> GSHMSDNPKVLVADDDKKIAQFIKTKFEENGIDTTVAFDGKEALFLINTNNYDVIVIDWMMPYLDGISLLKILRKQNINTPVIILSALDSTENKIEGLKSGSDDYLTKPFSID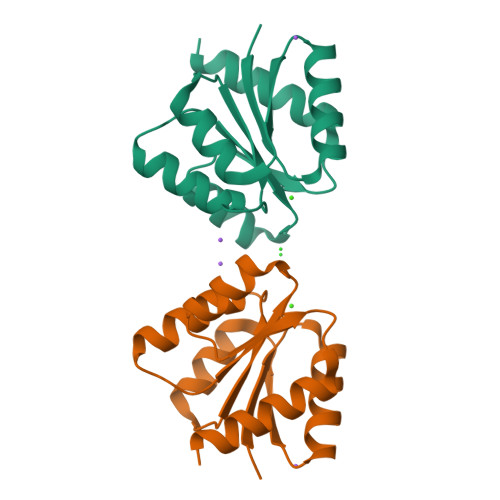ELIIRVNILYKRTKQITEA> MKTQVAIIGAGPSGLLLGQLLHKAGIDNVILERQTPDYVLGRIRA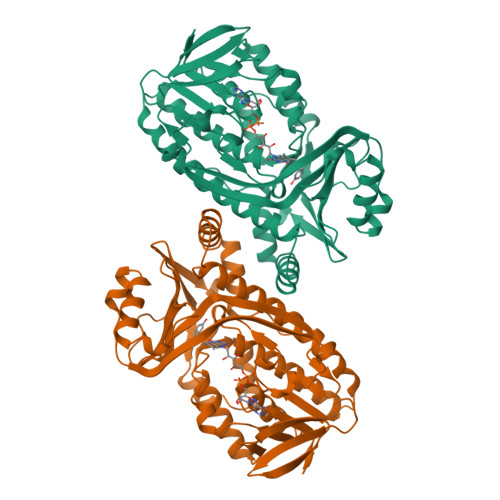GVLEQGMVDLLREAGVDRRMARDGLVHEGVEIAFAGQRRRIDLKRLSGGKTVTVYGQTEVTRDLMEAREASGATTVYQAAEVRLHDLQGERPYVTFERDGERLRLDCDYIAGCDGFHGISRQSIPAERLKVFERVYPFGWLGLLADTPPVSHELIYANHPRGFALCSQRSATRSRYYVQVPLTEKVEDWSDERFWTELKARLPAEVAEKLVTGPSLEKSIAPLTSFVVEPMQHGRLFLAGDAAHIVPPTGAKGLNLAASDVSTLYRLLLKAYREGRGELLERYSAICLRRIWKAERFSWWMTSVLHRFPDTDAFSQRIQQTELEYYLGSEAGLATIAENYVGLPYEEIE> MALRWGIVSVGLISSDFTAVLQTLPRSEHQVVAVAARDLSRAKEFAQKHDIPKAYGSYEELAKDPNVEVAYVGTQHPQHKAAVMLCLAAGKAVLCEKPMGVNAAEVREMVTEARSRGLFLMEA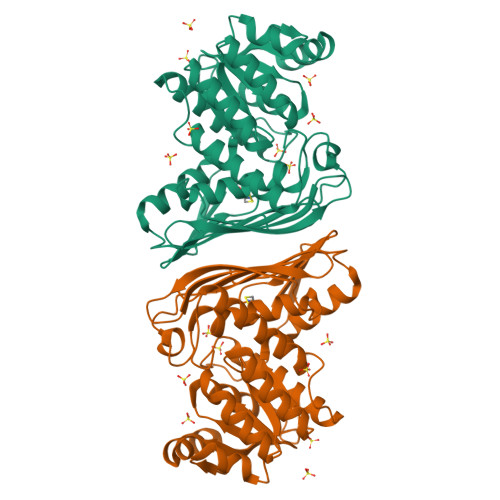IWTRFFPASEALRSVLAQGTLGDLRVARAEFGKNLTHVPRAVDWAQAGGALLDLGIYCVQFISMVFGGQKPEKISVMGRRHETGVDDTVTVLLQYPGEVHGSFTCSITAQLSNTASVSGTKGMAQLLNPCWCPTELVVKGEHKEFLLPPVPKNCNFDNGAGMSYEAKHVRECLRKGLKESPVIPLVESELLADILEEVRRAIGVTFPQDKH(7S)-2-[(3,5-difluoro-4-hydroxyphenyl)amino]-7-methyl-8-(3-methylbutyl)-5-(prop-2-yn-1-yl)-7,8-dihydropteridin-6(5H)-one | C21 H23 F2 N5 O2 | 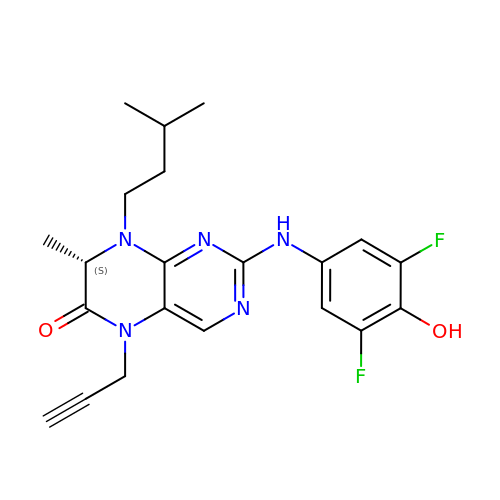IHZPRIAIJQSUAF-ZDUSSCGKSA-N>[2x]GSVEEI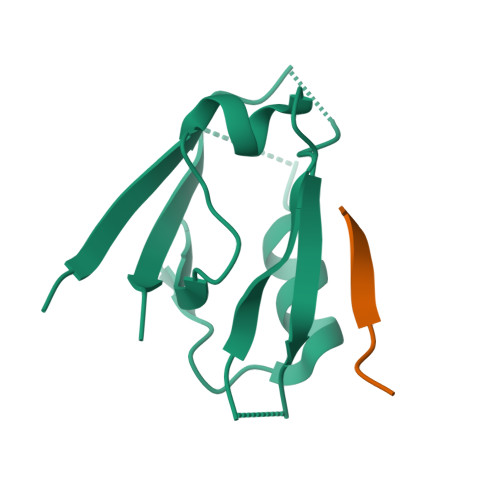RLPRAGGPLGLSIVGGSDHSSHPFGVQEPGVFISKVLPRGLAARSGLRVGDRILAVNGQDVRDATHQEAVSALLRPCLELSLLVRRD;>KHFRETEV[2x]>[4x]GPGSSLSRFRGCLAGALLGDCVGSFYAAHDTVDLTSVLRHVQSLEPDPGTPGSERTEALYYTDDTAMARALVQSLLAKEAFDEVDMAHRFAQEYKKDPDRGYGAGVVTVFKKLLNPKCRDVFEPARAQFNGKGSYGNGGAMRVAGISLAYSSVQDVQKFARLSAQLTHASSLGYNGAILQALAVHLALQGESSSEHFLKQLLGHMEDLEGDAQSVLDARELGMEERPYSSRLKKIGELLDQASVTREEVVSELGNGIAAFESVPTAIYCFLRCMEPDPEIPSAFNSLQRTLIYSISLGGDTDTIATMAGAIAGAYYGMDQVPESWQQSCEGYEETDILAQSLHRVFQKS

Poly(ADP-ribose)glycohydrolase (PARG) and (ADP-ribosyl)hydrolase 3 (ARH3) are the main hydrolases of serine PAR- and MARylation, respectively, thus playing a pivotal role in signal silencing following DNA damage. ARH3 is the only known enzyme to reverse serine MARylation and is consequently responsible for the regulation of hundreds of ADP-ribosylated proteins following DNA damage. In contrast to PARG, the active site of ARH3 contains a catalytic binuclear magnesium centre. To understand the impact of the ARH3:substrate interaction on reaction efficiency, we crystallised ARH3 in complex with the chemically synthesised substrates: histone H2B peptide (aa 1–11) MARylated on Ser7 (H2BS7mar), dimeric ADP-ribose (dimer) and α-NAD+.

Therefore, we chose to crystallise the hARH3 E41A substrate complexes as this prevents substrate cleavage during crystal formation, while retaining a functionally relevant magnesium coordination. Interestingly, while we observe an open conformation in the H2BS7mar- and α-NAD+-bound structures, both the hARH3:dimer and LchARH3:meADPr complexes adopt a closed conformation. In contrast, the ADPra1:n unit of the dimer binds in a relaxed conformation within the ligand site, which prevents engagement of the scissile bond with the Mg2+ ions. Similar to the peptide substrate, the ADPra1:n-1 makes only water-mediated contacts with the protein. The axial position of MgII is occupied by a water molecule (w610) due to the E41A mutation that was introduced to allow crystallisation. However, the protein backbone adopts a closed conformation, and our models suggest an interaction between Glu41 and MgII is possible. Within our hARH3:dimer structure, crystal packing does not impact the positioning of the ADPra1:n-1 moiety. Both ADPr groups of the dimeric PAR adopt a relaxed conformation and do not engage with the MgII centre to displace Glu41. The most likely reason for this unproductive binding mode is the strained position the ADPra1:n-1 would need to adopt as well as the lack of a further coordination groups (like the serine backbone carbonyl) to stabilise the binding. Yet PAR binding fails to efficiently induce these structural in ARH3, thus providing a structural explanation for the observed low hydrolytic activity towards this substrate.>GPHMLEAEHPLQYNYTFWYSRRTPGRPTSSQSYEQNIKQIGTFASVEQFWRFYSHMVRPGDLTGHSDFHLFKEGIKPMWEDDANKNGGKWIIRLRKGLASRCWENLILAMLGEQFMVGEEICGAVVSVRFQEDIISIWNKTASDQATTARIRDTLRRVLNLPPNTIMEYKTHTDSIKMPGRLGPQRLLF[2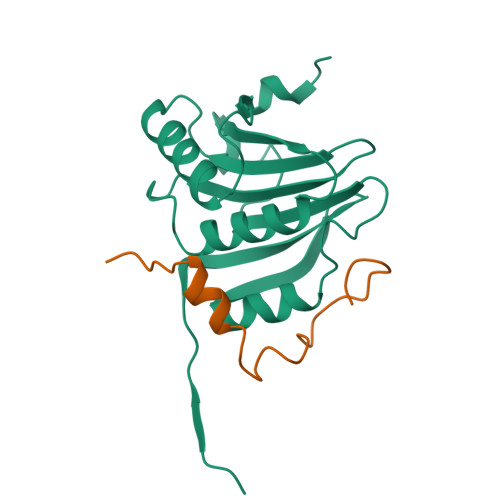x];>[2x]GPHMTRIIYDRKFLMECRNSPVTKTPPRDLPTIPGVTS4-methylsulfanylbenzoic acid | C8 H8 O2 S | 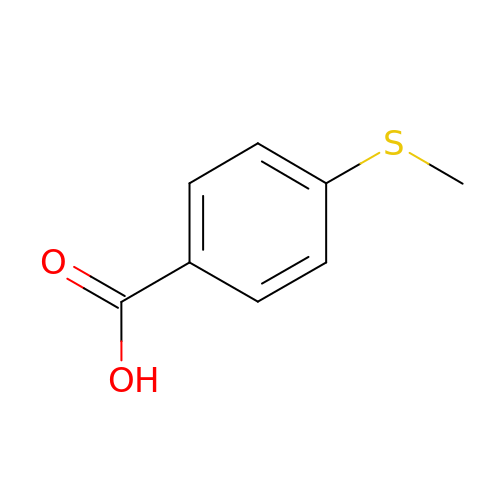KWHCPERWLHBLOT-UHFFFAOYSA-N> SMMELRVGNRYRLGRKIGSGSFGDIYLGTDIAAGEEVAI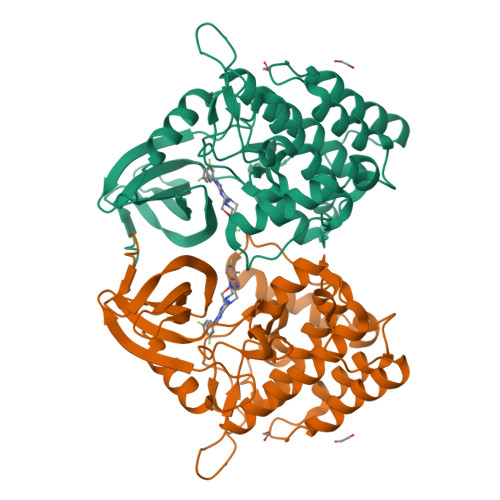KLECVKTKHPQLHIESKIYKMMQGGVGIPTIRWCGAEGDYNVMVMELLGPSLEDLFNFCSRKFSLKTVLLLADQMISRIEYIHSKNFIHRDVKPDNFLMGLGKKGNLVYIIDFGLAKKYRDARTHQHIPYRENKNLTGTARYASINTHLGIEQSRRDDLESLGYVLMYFNLGSLPWQGLKAATKRQKYERISEKKMSTPIEVLCKGYPSEFATYLNFCRSLRFDDKPDYSYLRQLFRNLFHRQGFSYDYVFDWNMLK>[2x]MSLVLNDLLICCRQLEHDRATERKKEVEKFKRLIRDPETIKHLDRHSDSKQGKYLNWDAVFRFLQKYIQKETECLRIAKPNVSASTQASRQKKMQEISSLVKYFIKCANRRAPRLKCQELLNYIMDTVKDSSNGAIYGADCSNILLKDILSVRKYWCEISQQQWLELFSVYFRLYLK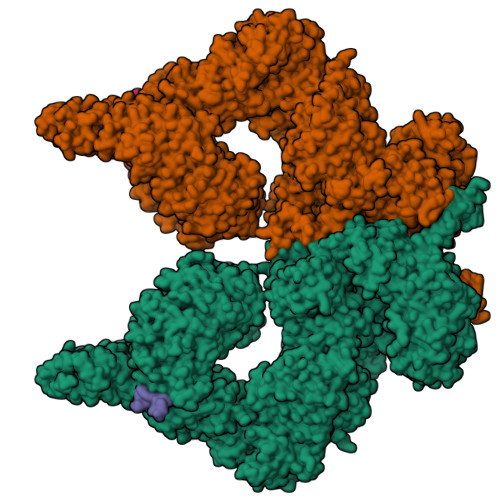PSQDVHRVLVARIIHAVTKGCCSQTDGLNSKFLDFFSKAIQCARQEKSSSGLNHILAALTIFLKTLAVNFRIRVCELGDEILPTLLYIWTQHRLNDSLKEVIIELFQLQIYIHHPKGAKTQEKGAYESTKWRSILYNLYDLLVNEISHIGSRGKYSSGFRNIAVKENLIELMADICHQVFNEDTRSLEISQSYTTTQRESSDYSVPCKRKKIELGWEVIKDHLQKSQNDFDLVPWLQIATQLISKYPASLPNCELSPLLMILSQLLPQQRHGERTPYVLRCLTEVALCQDKRSNLESSQKSDLLKLWNKIWCITFRGISSEQIQAENFGLLGAIIQGSLVEVDREFWKLFTGSACRPSCPAVCCLTLALTTSIVPGTVKMGIEQNMCEVNRSFSLKESIMKWLLFYQLEGDLENSTEVPPILHSNFPHLVLEKILVSLTMKNCKAAMNFFQSVPECEHHQKDKEELSFSEVEELFLQTTFDKMDFLTIVRECGIEKHQSSIGFSVHQNLKESLDRCLLGLSEQLLNNYSSEITNSETLVRCSRLLVGVLGCYCYMGVIAEEEAYKSELFQKAKSLMQCAGESITLFKNKTNEEFRIGSLRNMMQLCTRCLSNCTKKSPNKIASGFFLRLLTSKLMNDIADICKSLASFIKKPFDRGEVESMEDDTNGNLMEVEDQSSMNLFNDYPDSSVSDANEPGESQSTIGAINPLAEEYLSKQDLLFLDMLKFLCLCVTTAQTNTVSFRAADIRRKLLMLIDSSTLEPTKSLHLHMYLMLLKELPGEEYPLPMEDVLELLKPLSNVCSLYRRDQDVCKTILNHVLHVVKNLGQSNMDSENTRDAQGQFLTVIGAFWHLTKERKYIFSVRMALVNCLKTLLEADPYSKWAILNVMGKDFPVNEVFTQFLADNHHQVRMLAAESINRLFQDTKGDSSRLLKALPLKLQQTAFENAYLKAQEGMREMSHSAENPETLDEIYNRKSVLLTLIAVVLSCSPICEKQALFALCKSVKENGLEPHLVKKVLEKVSETFGYRRLEDFMASHLDYLVLEWLNLQDTEYNLSSFPFILLNYTNIEDFYRSCYKVLIPHLVIRSHFDEVKSIANQIQEDWKSLLTDCFPKILVNILPYFAYEGTRDSGMAQQRETATKVYDMLKSENLLGKQIDHLFISNLPEIVVELLMTLHEPANSSASQSTDLCDFSGDLDPAPNPPHFPSHVIKATFAYISNCHKTKLKSILEILSKSPDSYQKILLAICEQAAETNNVYKKHRILKIYHLFVSLLLKDIKSGLGGAWAFVLRDVIYTLIHYINQRPSCIMDVSLRSFSLCCDLLSQVCQTAVTYCKDALENHLHVIVGTLIPLVYEQVEVQKQVLDLLKYLVIDNKDNENLYITIKLLDPFPDHVVFKDLRITQQKIKYSRGPFSLLEEINHFLSVSVYDALPLTRLEGLKDLRRQLELHKDQMVDIMRASQDNPQDGIMVKLVVNLLQLSKMAINHTGEKEVLEAVGSCLGEVGPIDFSTIAIQHSKDASYTKALKLFEDKELQWTFIMLTYLNNTLVEDCVKVRSAAVTCLKNILATKTGHSFWEIYKMTTDPMLAYLQPFRTSRKKFLEVPRFDKENPFEGLDDINLWIPLSENHDIWIKTLTCAFLDSGGTKCEILQLLKPMCEVKTDFCQTVLPYLIHDILLQDTNESWRNLLSTHVQGFFTSCLRHFSQTSRSTTPANLDSESEHFFRCCLDKKSQRTMLAVVDYMRRQKRPSSGTIFNDAFWLDLNYLEVAKVAQSCAAHFTALLYAEIYADKKSMDDQEKRSLAFEEGSQSTTISSLSEKSKEETGISLQDLLLEIYRSIGEPDSLYGCGGGKMLQPITRLRTYEHEAMWGKALVTYDLETAIPSSTRQAGIIQALQNLGLCHILSVYLKGLDYENKDWCPELEELHYQAAWRNMQWDHCTSVSKEVEGTSYHESLYNALQSLRDREFSTFYESLKYARVKEVEEMCKRSLESVYSLYPTLSRLQAIGELESIGELFSRSVTHRQLSEVYIKWQKHSQLLKDSDFSFQEPIMALRTVILEILMEKEMDNSQRECIKDILTKHLVELSILARTFKNTQLPERAIFQIKQYNSVSCGVSEWQLEEAQVFWAKKEQSLALSILKQMIKKLDASCAANNPSLKLTYTECLRVCGNWLAETCLENPAVIMQTYLEKAVEVAGNYDGESSDELRNGKMKAFLSLARFSDTQYQRIENYMKSSEFENKQALLKRAKEEVGLLREHKIQTNRYTVKVQRELELDELALRALKEDRKRFLCKAVENYINCLLSGEEHDMWVFRLCSLWLENSGVSEVNGMMKRDGMKIPTYKFLPLMYQLAARMGTKMMGGLGFHEVLNNLISRISMDHPHHTLFIILALANANRDEFLTKPEVARRSRITKNVPKQSSQLDEDRTEAANRIICTIRSRRPQMVRSVEALCDAYIILANLDATQWKTQRKGINIPADQPITKLKNLEDVVVPTMEIKVDHTGEYGNLVTIQSFKAEFRLAGGVNLPKIIDCVGSDGKERRQLVKGRDDLRQDAVMQQVFQMCNTLLQRNTETRKRKLTICTYKVVPLSQRSGVLEWCTGTVPIGEFLVNNEDGAHKRYRPNDFSAFQCQKKMMEVQKKSFEEKYEVFMDVCQNFQPVFRYFCMEKFLDPAIWFEKRLAYTRSVATSSIVGYILGLGDRHVQNILINEQSAELVHIDLGVAFEQGKILPTPETVPFRLTRDIVDGMGITGVEGVFRRCCEKTMEVMRNSQETLLTIVEVLLYDPLFDWTMNPLKALYLQQRPEDETELHPTLNADDQECKRNLSDIDQSFNKVAERVLMRLQEKLKGVEEGTVLSVGGQVNLLIQQAIDPKNLSRLFPGWKAWV;>[2x]MEVQNQHAKEESLADDLFRYNPYLKRRR> ALETLAFDGRTYIEYLNAVIESELTNEIPAEKALQSNHFELSLRTEATQGLVLWIGKAAERADYMALAIVDGHLQLSYDLGSQPVVLRSTVKVNTNRWLRIRAHREHREGSLQVGNEAPVTGSSPLGATQLDTDGALWLGGLQKLPVGQALPKAYGTGFVGCLRDVVVGHRQLHLLE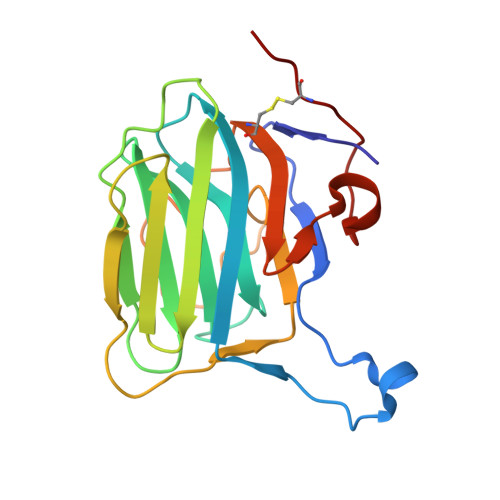DAVTKPELRPCPTP> MNKKSMKTVLGVAALSLLASCNSTYAPNVDSTVSLKGTDVFKADSASIAQNYTIPEWFKDAKFGIFIHWGVYSVPAYGSEWYSRWMYKEGHPINKYHVQTYGPLTKFGYKDFIPMFKAENFNADEWLAVVKSSGAQYIVPVAEHHDGFAMYSSTFNKWNAVDM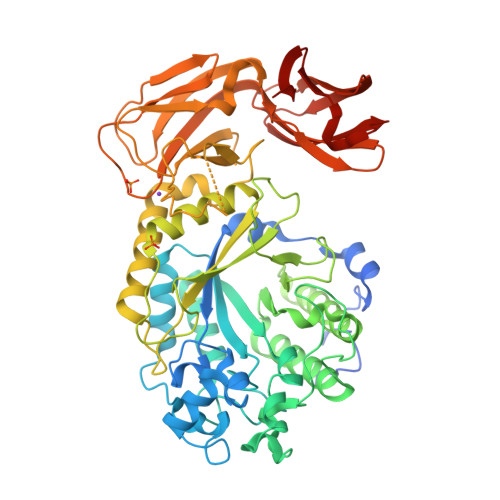GPKRDIIGELKEATKKAGLRFGLSSHRCENAWFYEYGMETPSDVQDTTITLYGERLHEPEGQGMTPYCGKYEGSNERSRRQFLMHTYELIDKYQPELIWFDWTVGKYPFQPTFYKFMAYYYNSALDWNKEVVVNTKFGYGDNIQVFDIERGKSDRIREYPWQTDTSVGKKSWSYCVGEENKSPDHIIDDFVDIVSKNGNLLLNIGPKADGTITDEQKNVLAEIGKWLKTNGEAIYGSRPWVIASEGHNAGTAGYMTDNTKTEYTADDIRFTTCDNNLYAVSLAWTDGSVTIKSLATKYCRNVEIESVEMLGSSEKIDYKMTDEGLVVNFPKNKPTEYAHVFKIKLKGVVVSKPLYDKVDNGCLITVRVANHNAEDANVTLKSVVDGNEVSTQVAVKAKSEQWVKMQNKDVKSFDDMSCKFYFNDNLTYENEFKK>MEPSSLELPADTVQRIAAELKCHPTDERVALHLDEEDKLRHFRECFYIPKIQDLPPVDLSLVNKDEDAIYFNGNSLGLQPKMVKTYLEEELDKWAKIAIYGWFEGDSPWIHYDESIVGLMKDIVGANEKEIVLMNTLTVNLHLLMLSFFKPTPKRYKILLEAKAFPSDHYAIESQLQLHGLNIEESMRIIKPREGEETLRIEDILEVIEKEGDSIAVILFSGIHYYTGQHFNIPAITKAGQAKGCYVGFDLAHAVGNVELYLHDWGVDFACWCGYKYLNSSPGGIAGAFIHEKHAHTIKPALVGWFGHELSTRFKMDNKLQLIPGVCGFRCSTPPILLVCILHASLEIFKQATMKALRKKSVLLTGYLEYLIKHNYGKDKAATKKPVVNIITPSHVEERGCQLTLTFNVPNKDVFQELEKRGVVCDKRNPNGIRVAPVPLYNSFHD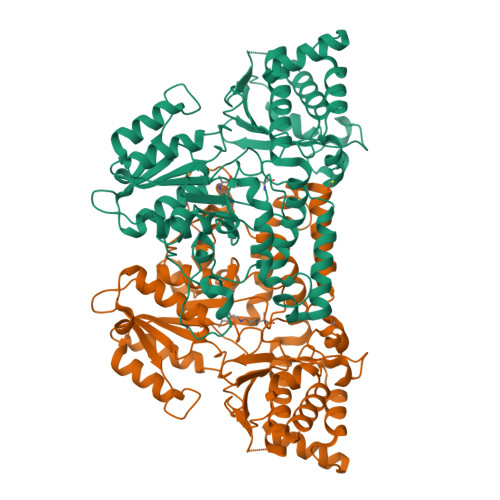VYKFTNLLTSILDSAETKN[2x]2-[(S)-(2-chlorophenyl){2-[(2R)-1-methylpyrrolidin-2-yl]ethoxy}methyl]-1H-pyrrolo[3,2-b]pyridine-7-carboxylic acid | 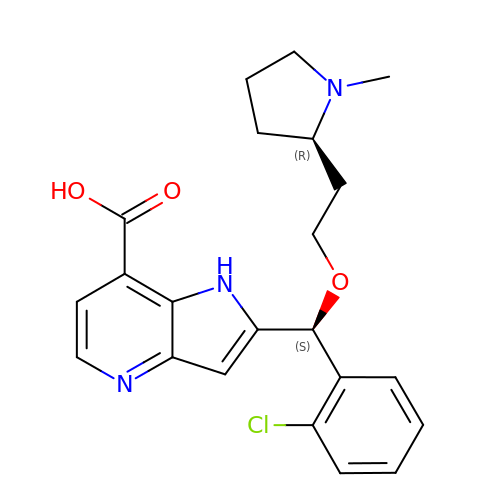C22 H24 Cl N3 O3 | FLCRYTPTFPDXRU-SZNDQCEHSA-N>[8x]MSGMRFDTRLVHGGRRPSAGTGDVVPPIHVSTTYERR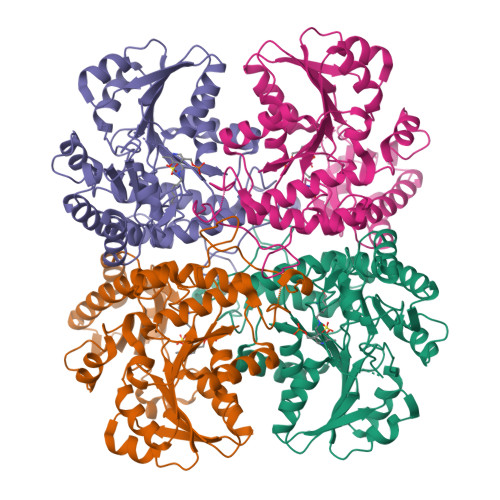AQDEPRYFYGRGENPTREELEECLAGLERAPFATVFSSGQAAAATLLSLVRPGQCVVSTDDVYAGTDGLFDLAARQGVRVRYADLTTPEGIAAALAEPDLALVWIETPTNPLLTVVDVAEVSRRAHERGARVVVDNTFASPVLQQPLALGADVSLYSTTKSIAGHADVLGGALVYRDADLHAAVRAYRTTAGNVPGALDCFLVRRGLHTLSLRVHRQVATARVLVERLRASPVVGAVHYPGLPEHPQHAVVKAQMSAPGAIVSFDYLGGPAERLLDRFTLFTCGVSLGGVHSLVECPALMTHRPLSAEARARRGIGESLIRLSVGIEDPQDLAEDLSRALAGGTLEHHHHHH>MLTPTERKRQGYIHELIVTEENYVNDLQLVTEIFQKPLMESELLTEKEVAMIFVNWKELIMCNIKLLKALRVRKKMSGELATTLERIEKNFVITDPRLPDNPIIFASDSFLQLTEYSREEILGRNMRFLQGPETDRATVRKIRDAIDNQTEVTVQLINYTKSGKKFWNLFHLQPMRDQKGDVQYFIGVQLDGTEHVRDAAEREGVMLIKKTAENIDEAAKELKMPVKMIGDILSAQLPHMQPYIRFCSRQLNGAALIQQKTDEAPDFKEFVKRLAMDPRCKGMPLSSFILKPMQRVTRYPLIIKNILENTPENHPDHSHLKHALEKAEELCSQVNEGVREKENSDRLEWIQAHVQCEGLSEQLVFNSVTN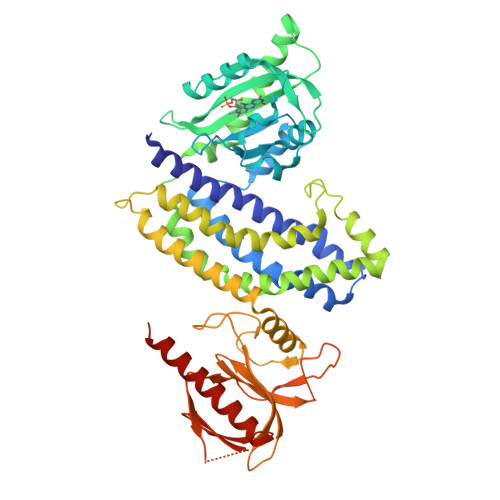CLGPRKFLHSGKLYKAKSNKELYGFLFNDFLLLTQITKPLGSSGTDKVFSPKSNLQYKMYKTPIFLNEVLVKLPTDPSGDEPIFHISHIDRVYTLRAESINERTAWVQKIKAASELYIETEKKKLEHHHHHH[2x]>YVSESEPLVRFKNSVKITKGDLNSWREGTDPCSGKWFGIYCQKGLTVSGIHVTRLGLSGTI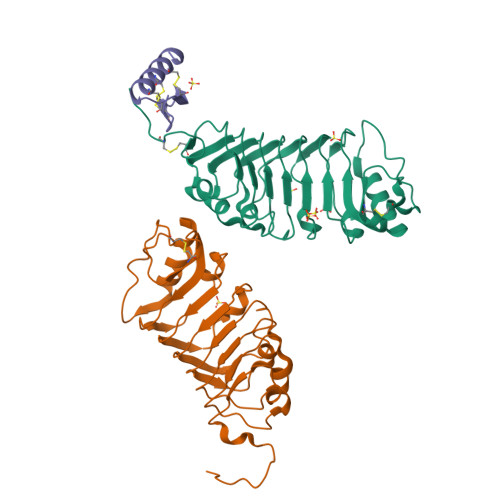TVDDLKDLPNLKTIRLDNNLLSGPLPHFFKLRGLKSLMLSNNSFSGEIRDDFFKDMSKLKRLFLDHNKFEGSIPSSITQLPQLEELHMQSNNLTGEIPPEFGSMKNLKVLDLSTNSLDGIVPQSIADKKNLAVNLTENEYLCGPVVDVGCENIELNDPQEGQPPSKPSSSVPETSHHHHHH[2x];> TLINGSSDEERTYSFSPTTSPFDPRSLNQELKIGRIGYCFDCARACMRRGKYIRTCSFERKLCRCSISDIK>AAPTAIEHMEPPFWWAGMQHKGLQLMVHGRDIGRMEAALDYPGVRLVSPTRVPNANYLFVDLEIGPEAQPGSFDIVFKGDGRSERYRYRLLAREQGSAQRQGFGPGDAIYQIMPDRFANGDPSND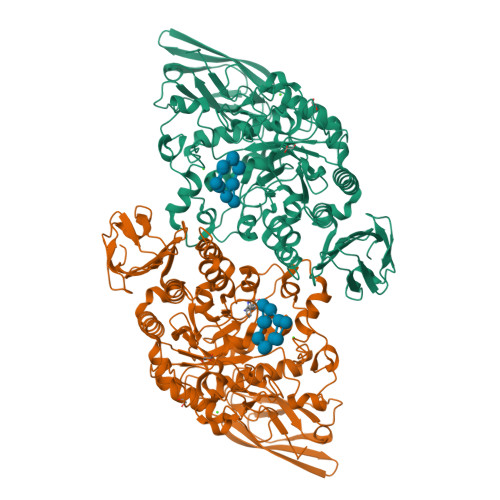NVAGMREQADRRHGGGRHGGDIRGTIDHLDYIAGLGFTQLWPTPLVENDAAAYSYHGYAATDHYRIDPRYGSNEDFVRLSTEARKRGMGLIQDVVLSHIGKHHWWMKDLPTPDWINYGGKFVPTQHHRVAVQDPYAAQADSENFTKGWFVEGMPDLNQTNPLVANYLIQNNIWWIEYAGLSGLRIDTYGYSDGAFLTEYTRRLMAEYPRLNMVGQEWSTRVPVVARWQRGKANFDGYTSHLPSLMDFPLVDAMRNALSKTGEENGLNEVYETLSLDYLYPEPQNLVLFGGNHDMARMFSAAGEDFDRWRMNLVFLMTMPRIPQFYSGDEILMTSTVKGRDDASYRRDFPGGWAGDKANAFSGAGLTSQQRAAQDLVRKLANWRKNQPVIHNGRLMHFGPEENTWVYFRYNKDKRIMVAMNNNDKPMTLPTARFQEMLKGAPSGVDFLSGKTVGLGRELRLAPKSVVVIELPGLPEA[2x]>[2x]MSTQYETQGYTINNAGRRLVVDPITRIEGHMRCEVNINDQNVITNAVSCGTMFRGLEIILQGRDPRDAWAFVERICGVCTGVHALASVYAIEDAIGIKVPDNANIIRNIMLATLWCHDHLVHFYQLAGMDWIDVLDALKADPRKTSELAQSLSSWPKSSPGYFFDVQNRLKKFVEGGQLGIFRNGYWGHPQYKLPPEANLMGFAHYLEALDFQREIVKIHAVFGGKNPHPNWIVGGMPCAINIDESGAVGAVNMERLNLVQSIITRTADFINNVMIPDALAIGQFNKPWSEIGTGLSDKCVLSYGAFPDIANDFGEKSLLMPGGAVINGDFNNVLPVDLVDPQQVQEFVDHAWYRYPNDQVGRHPFDGITDPWYNPGDVKGSDTNIQQLNEQERYSWIKAPRWRGNAMEVGPLARTLIAYHKGDAATVESVDRMMSALNLPLSGIQSTLGRILCRAHEAQWAAGKLQYFFDKLMTNLKNGNLATASTEKWEPATWPTEC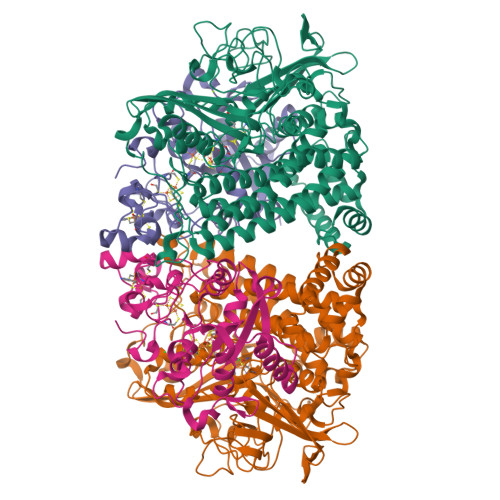RGVGFTEAPRGALGHWAAIRDGKIDLYQCVVPTTWNASPRDPKGQIGAYEAALMNTKMAIPEQPLEILRTLHSFDPCLACSTH;>[2x]LENKPRIPVVWIHGLECTCCTESFIRSAHPLAKDVILSLISLDYDDTLMAAAGTQAEEVFEDIITQYNGKYILAVEGNPPLGEQGMFCISSGRPFIEKLKRAAAGASAIIAWGTCASWGCVQAARPNPTQATPIDKVITDKPIIKVPGCPPIPDVMSAIITYMVTFDRLPDVDRMGRPLMFYGQRIHDKCYRRAHFDAGEFVQSWDDDAARKGYCLYKMGCKGPTTYNACSSTRWNDGVSFPIQSGHGCLGCAENGFWDRGSFYSRGSFYSRHHHHHH>[2x]MTSPSHASDRGGGDGDSVENQSPELRKDPVTNRWVIFSPARAKRPTDFKSKSPQNPNPKPSSCPFCIGREQECAPELFRVPDHDPNWKLRVIENLYPALSRNLETQSTQPETGTSRTIVGFGFHDVVIESPVHSIQLSDIDPVGIGDILIAYKKRINQIAQHDSI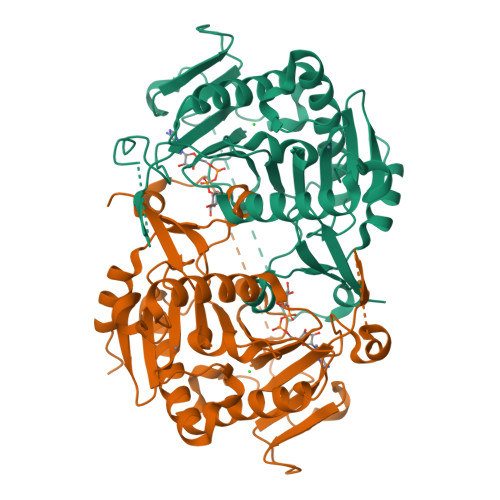NYIQVFKNQGASAGASMSHSGSQMMALPVVPPTVSSRLDGTKDYFEETGKCCLCEAKSKHFVIDESSHFVSVAPFAATYPFEIWIIPKDHSSHFHHLDDVKAVDLGGLLKLMLQKIAKQLNDPPYNYMIHTSPLKVTESQLPYTHWFLQIVPQLSGVGGFEIGTGCYINPVFPEDVAKVMREVSLT SULFUR DIOXIDE | 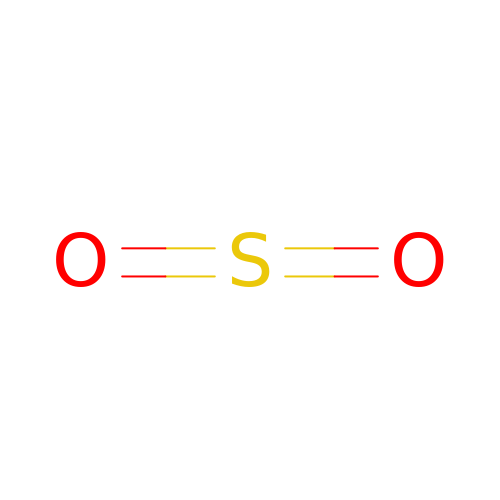O2 S | RAHZWNYVWXNFOC-UHFFFAOYSA-N> MQYSIEKLKKEENSLAKDYYIYRLLEKNKISKKDAQDLQSHIFRYIGKIKSELEKIIPLKPYINPKYAKCYTYTANTILDANLTCQSVRLNSLVFIASLNSKDRTTLAQTFKNQRPDLTNLLL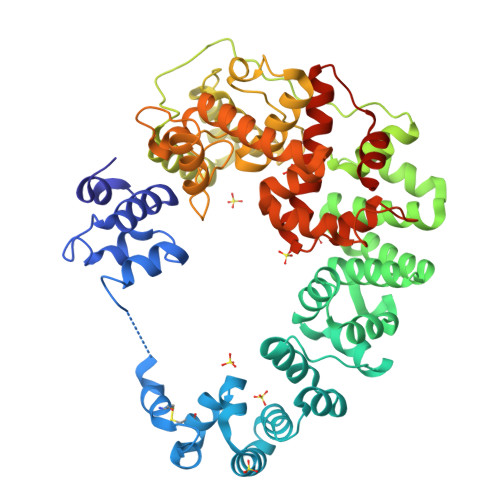AFNTSDPMSYIVQKEDINGFFKLYNYSKKYDLDLNTSLVNKLPNHIGFKDFAQNIIIKKENPKFRHSMLEINPENVSEDSAFYLGVNALTYDKTELAYDFFKKAAQSFKSQSNKDNAIFWMWLIKNNEEDLKTLSQSSSLNIYSLYAKELTNTPFPKIESLNPSKKKNNFNMQDPFAWQKINKQIRDANASQLDVLAKEFDTQETLPIYAYILERKNNFKKHYFIMPYYDNIKDYNKTRQALILAIARQESRFIPTAISVSYALGMMQFMPFLANHIGEKELKIPNFDQDFMFKPEIAYYFGNYHLNYLESRLKSPLFVAYAYNGGIGFTNRMLARNDMFKTGKFEPFLSMELVPYQESRIYGKKVLANYIVYRHLLNDSIKISDIFENLIQNKANDLNKS1-nitropropane | C3 H7 N 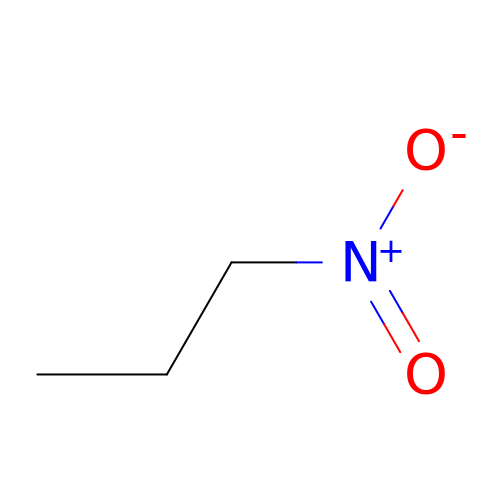O2 | JSZOAYXJRCEYSX-UHFFFAOYSA-N>MGSDKIHHHHHHMSAVTESVLESIISPVTMSEFLEEYWPVKPLVARGEVERFTSIPGFEKVRTLENVL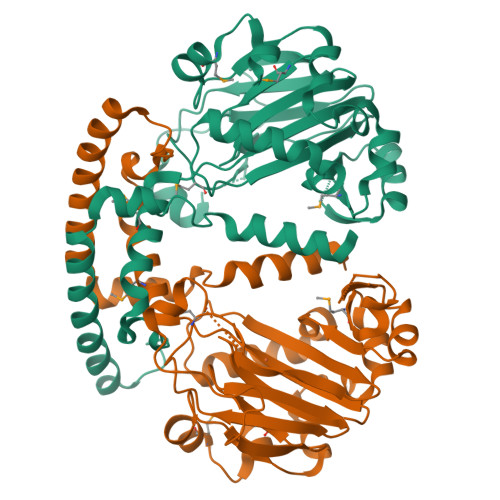AIYNNPVMVVGDAVIEESEGITDRFLVSPAEALEWYEKGAALEFDFTDLFIPQVRRWIEKLKAELRLPAGTSSKAIVYAAKNGGGFKAHFDAYTNLIFQIQGEKTWKLAKNENVSNPMQHYDLSEAPYYPDDLQSYWKGDPPKEDLPDAEIVNLTPGTMLYLPRGLWHSTKSDQATLALNITFGQPAWLDLMLAALRKKLISDNRFRELAVNHQSLHESSKSELNGYLESLIQTLSENAETLTPEQIFQSQDSDFDPYQSTQLVFRQLLTSYKF[4x]> SNAMSVQTIERLQDYLLPEWVSIFDIADFSGRMLRIRGDIRPALLRLASRLAELLNESPGPRPWYPHVASHMRRRVNPPPETWLALGPEKRGYKSYAHSGVFIGGRGLSVRFILKDEAIEERKNLGRWMSRSGPAFEQWKKKVGDLRDFGPVHDDPMADPPKVEWDPRVFGERLGSLKS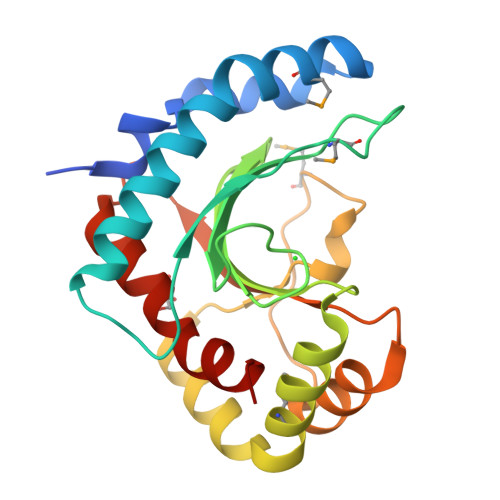ASLDIGFRVTFDTSLAGIVKTIRTFDLLYAEAEKGS>GPERTFIMVKPDGVQRGLVGEVIQRFERRGYKLVAIKMMHASEQLLQTHYEALKSLSFFPKLVAYMSSGPVVPMVFEGRKVVENGRTMLGATKPEASCPGSIRGDYCQDVGRNVVHGSDSTESANREINLW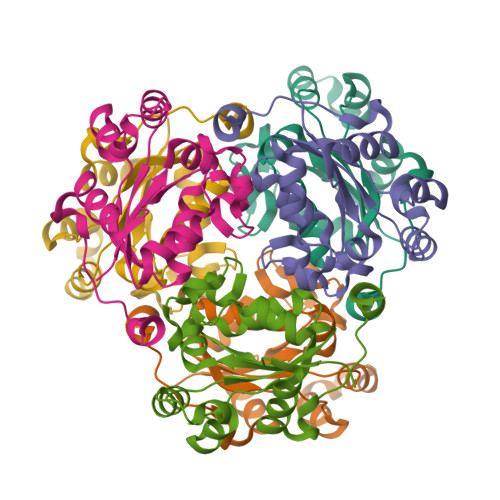FSPQELCQYKQAVDPWIHE[12x]>[2x]GSNRMTEMHVCLADAIQKDNRPEISNRLFRSNAVEKEILRVQKLLKNAKLAWMFTNCFPNTLDTTV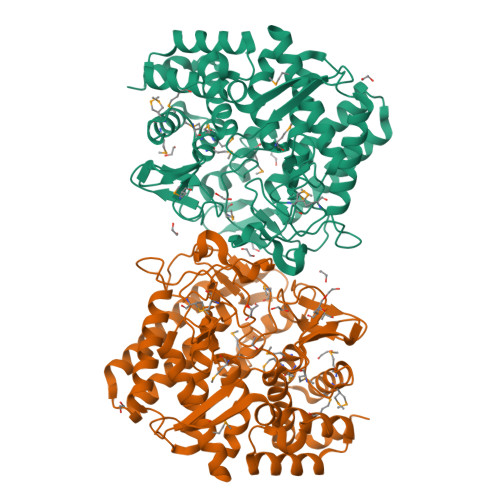HFRKGSDGKPDTFVYTGDIHAMWLRDSGAQVWPYVQLANSDPELKEMLAGVILRQFKCINIDPYANAFNDGAIPDGHWMSDLTDMKPELHERKWEIDSLCYPLRLAYHYWKTTGDASIFNEEWIQAITNVLKTFKEQQRKDGVGPYKFQRKTERALDTVSNDGLGAPVKPVGLIVSSFRPSDDATTLQFLVPSNFFAVSSLRKAAEILEKVNKKTALSKECKDLAQEVETALKKYAVYNHPKYGKIYAFEVDGFGNHHLMDDANVPSLLAMPYLGDVNVNDPIYQNTRRFVWSEDNPYFFKGKAGEGIGGPHIGYDMVWPMSIMMKAFTSQNDAEIKTCIKMLMDTDAGTGFMHESFHKDNPKKFTRAWFAWQNTLFGELILKLVNEGKVDLLNSIQ>MTDMISAPWEASLTQAEHSLIFYFLALTGSALLFGLARTWLTRGEVGARYRTAVVARSGIMIVATLSYVFMVLAFTSGYDHVGSLWVPNSEAIMTIAPRYVEWSIAVPLLSIELLSVATLSGVSARRTRLAAVAGAFLMIFTGFLGAVVIGDGRSVGSLIIWGAISTVFWIITAVILIRAIRHSLPQLTPEAAALLKTATIFLMSGWAVYPLAYLIQILFAGGLWTTSIHIILCTADIVVKLGFCGLIHRIAKLRTAEDVRAGVDIHTEAIWISSVKQSDAGIPTVVYLPEGETIHQRRPKPSDSNATASSSARQWTDDFPPTDL[5x]

Here, we describe a rhodopsin group found in microorganisms from cold environments, such as glaciers, denoted as CryoRhodopsins (CryoRs). A distinguishing feature of the group is the presence of a buried arginine residue close to the cytoplasmic face. Combining single-particle cryo–electron microscopy and x-ray crystallography with rhodopsin activation by light, we demonstrate that the arginine stabilizes an ultraviolet (UV)–absorbing intermediate of an extremely slow CryoRhodopsin photocycle. Our data suggest that CryoRs are sensors for UV irradiation and are also capable of inward proton translocation modulated by UV light.

Among the studied CryoRs, CryoR1 shows several unique spectroscopic features, both in steady-state and time-resolved experiments. Notably, one rhodopsin (CryoR1 from Cryobacterium levicorallinum) has several absorption maxima over a wide range of pH values and showed a 80-nm red shift to 620 nm below pH 6. Specifically, at pH < 6, the spectrum is dominated by the red-shifted band at 620 nm. In contrast to many known MRs, the pH-dependent spectral shift of CryoR1 is not observed in a continuous movement across the spectral range but rather in a gradual decrease of the red-shifted absorption maximum at 620 nm associated with a rise of the blue-shifted absorption maximum at 540 to 550 nm and the deprotonated RSB band (400 nm). Furthermore, CryoR1 exhibits strong coherent oscillations on the ultrafast timescale in its 620-nm absorbing state at low pH indicating a hindered isomerization of the retinal chromophore. The strength of the coherent oscillations suggests a hindered retinal isomerization after excitation, in agreement with the extremely small signal amplitudes of the K state. Therefore, the unique large spectral shift shown for CryoR1 cannot be simply described by the protonation of the RSB counterions, and the molecular basis of this shift is further described in the “Protonation states of the counterions in CryoRs” section of the Supplementary Text.6-CHLORO-4-(CYCLOHEXYLSULFINYL)-3-PROPYLQUINOLIN-2(1H)-ONE 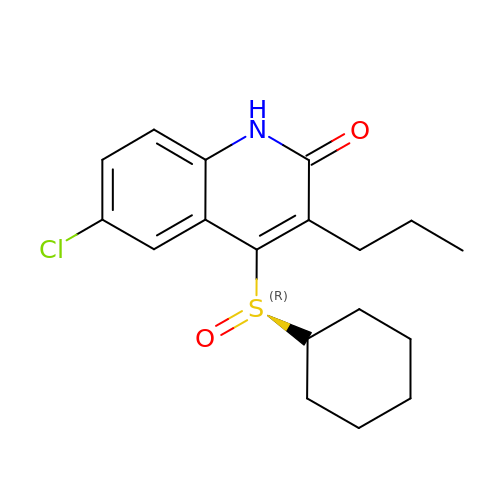| C18 H22 Cl N O2 S | QRBUGQMJMFAHKS-HSZRJFAPSA-N>MNITQAAEQAIRLWFNTPDPMQRLHMAKTIRTWIRQDKFAQVDQANMPNCVQQILNIIYDGLKPQPVQLPISYYAQLWYNLLDILRRFTFLPIISPYIHQVVQMFCPRENGPQDFRELICNLISLNWQKDPHMKHCANQVFQIFNCIIMGVKNEKLRTEFAQHLKFEKLVGTLSEYFNPQVHPGMINPAIFIIFRFIISKDTRLKDYFIWNNNPHDQPPPPTGLIIKLNAVMIGSYRLIAGQNPETLPQNPELAHLIQVIIRTFDLLGLLLHDSDAIDGFVRSDGVGAITTVVQYPNNDLIRAGCKLLLQVSDAKALAKTPLENILPFLLRLIEIHPDDEVIYSGTGFLSNVVAHKQHVKDIAIRSNAIFLLHTIISKYPRLDELTDAPKRNRVCEIICNCLRTLNNFLMMWIPTPNGETKTAGPNEKQQVCKFIEIDILKKLMSCLSCEGMDTPGLLELRSTILRSFILLLRTPFVPKDGVLNVIDENRKENLIGHICAAYSWVFRQPNNTRTQSTKQQLVERTISLLLVLMEQCGAEKEVAQYSYSIDCPLNLLNGNQVKPTFIHNVLVVCDKILEHCPTRADIWTIDRPMLEGLTNHRNSDIAKAAN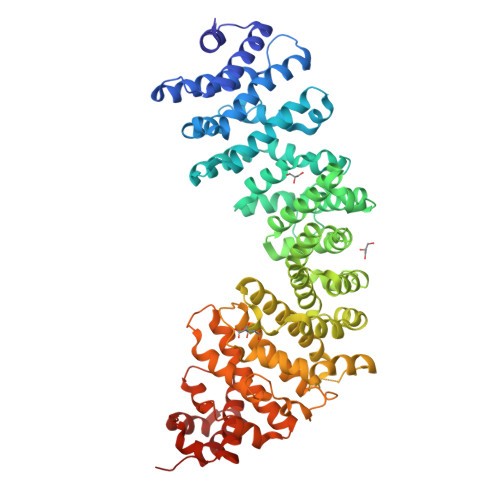SLLSRFPEN[2x]>MALRACGLIIFRRCLIPKVDNNAIEFLLLQASDGIHHWTPPKGHVEPGEDDLETALRETQEEAGIEAGQLTIIEGFKRELNYVARNKPKTVIYWLAEVKDYDVEIRLSHEHQAYRWLGLEEACQLAQFKEMKAALQEGHQFLCS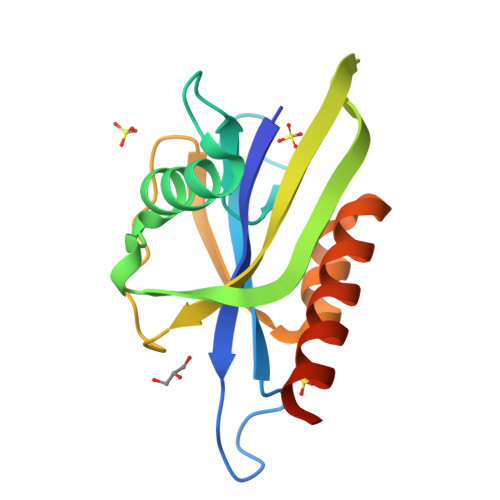IEALEHHHHHH[4x]2-morpholin-4-ylethyl 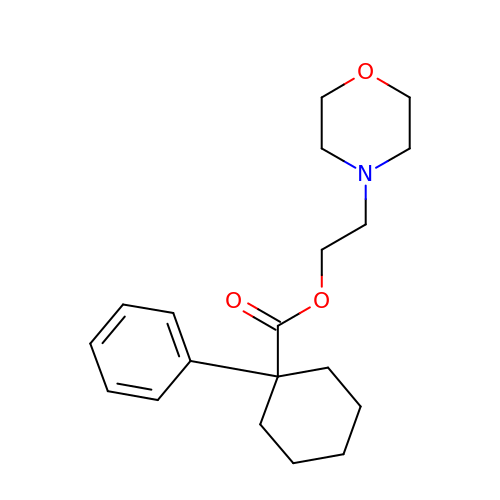1-phenylcyclohexane-1-carboxylate | C19 H27 N O3 | RQHKZUBCUZVZEF-UHFFFAOYSA-N> MKQKINKLLKNKGVQDKYKYLSKLILLDQEIKGKIKRKNKKEKQKRKNKLILEEMQNTTNIVHVPVHMGHTHYFDYIDSFPKLKEGPTLEENHITNQKILREQLISGQQGLEQNLCLRNCFKLSQKRYIE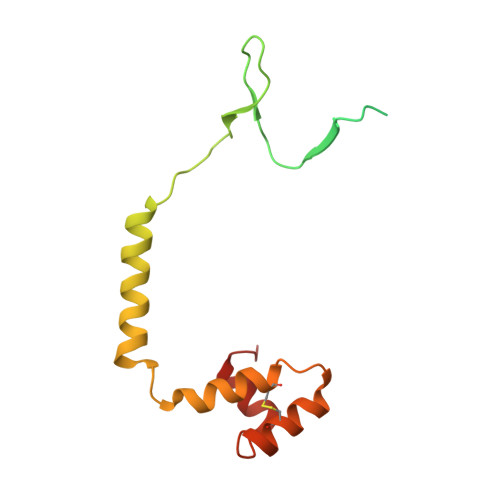FCLDRKCGGADFQRAATILGYTKN>[4x]MDEESASRASVPASSDREGAEFTRLPVSWTVNPRDAANARAAWKTLSAYHRGKPKSSRKLHVVYVTFKDRPALEGYRERYDHILKNIQAYYADQMQANGFPPLTFQLDLDERGKLVIHDAYVDKPMSEMSVQSSGPVSREAARKVLASKGIDIEKEHVLVVCQLPDGVGPYYGGGFSHQGTGWTCDQEGLDPASFLDTEMMQGGRFKVTRGKNATIYIGGTAHELGHSFGLPHTGDGWNYPDAGASLMGHGNSTYGDELRHEGKGAYLAPTDALKLASVPLFNGVETELPADASFGRMLGKYVPGSFERLEAIPVKDGLRLKGRVHLTRPAYGIVAHLDPPGGSDYDSNAVGASLDEKGEFDLTICRPGYKGGFIEMRVAVLNCDSTRSMITLPVWMDARGTKAPSLAQIVYFGDVQNLWIRGRTEEARKALAEVERRHGSRSEVKEWLPVWKRALGRQEPALEVVPAQIPAATASISLNDCKPSV

The uncharacterized protein AMUC_1438 is encoded by a gene that was previously shown to be upregulated when the bacterium is grown on mucin. Here, we provide structural and functional support for the assignment of AMUC_1438 as a unique O-glycopeptidase with mucin-degrading capacity. Structural, kinetic, and mutagenic analyses point to a metzincin metalloprotease catalytic motif but with an active site that specifically recognizes a GalNAc residue α-linked to serine or threonine (i.e., the Tn-antigen). The enzyme catalyzes hydrolysis of the bond immediately N-terminal to the glycosylated residue.

The core fold of the protein comprises a five-stranded β-sheet with a single α-helix packed on one face and region of multiple α-helices on the other face of the β-sheet. Pressed against this α-helical region is a β-sandwich domain comprising opposing four-stranded and three-stranded antiparallel β-sheets. Bound to the β-sandwich domain was a metal ion that was modeled as a calcium atom. A central feature of this catalytically active O-glycopeptidase fold is an ∼30 Å long helix that contains the HEXXH portion of the zinc-binding motif where the glutamate is the catalytic residue. The third histidine residue outside the canonical metallopeptidase motif, H233, completes the zinc-binding motif and is found on a loop structurally adjacent to the α-helix supporting the rest of the catalytic machinery. Underlying this is the “met-turn,” which places a methionine side chain directly beneath the zinc-binding site. Together, these features identify the catalytic center as having a metzincin motif. Overall, this fold is the same as that described for OgpA, the most structurally similar protein to ALT (RMSD of 2.1 Å, amino acid sequence identity of 19% over 292 aligned residues) and whose structure was described in detail previously. However, two tyrosine residues in ALT, Y171 and Y217, were structurally conserved with a phenylalanine and a tryptophan in OgpA, both of which are structurally implicated in glycan recognition in the G′ subsites of OgpA.>[4x]MDDASIDLQRAARDAAYSMPIEEINPADPELFRTDTMWPYFERLRKEDPVHWGVSPHEDVGGYWSVTKYNDIMAVDTNHEVFSSEPTIVLPDPADDFTLPMFIAMDPPKHDVQRKTVQPIVAPNHLAYLEPIIRERAGKILDDLPIGEEINWVDKVSIELTTMTLATLFDFPWEDRRKLTFWSDVATSAPESGILGTTDPEEHENLRRQTLFECVDYFMRLWN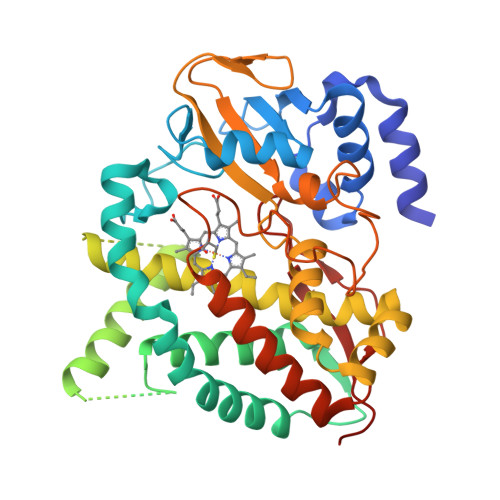ERVNAPPKPDLISMLAHGESTKNMDRMEYLGNLILLIVGGNDTTRNTISGSVLALHQNPDQDRKLRENPGLIPAMVSETIRWQTPLAYMRRRAKRDFELGGKTIREGDKVAMWYVSGNRDEEVIDRPNDYWIERPRVRQHLSFGFGVHRCVGNRLAELQLKIIWEEILARFPRLEVVGPPRRVYSSFVKGYEELPVVIPTRN>HHHHHHHHMKSESKVSSKLELRELVLLAMVI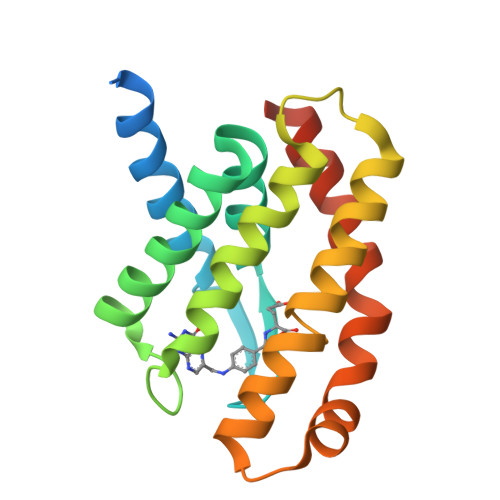AIKVVLGQFKVGDATLQVGLGFIGSVMLGYLFGPWWGFAGGALSDLVSSAIFGNLGGFFIGFTLTAALESMIYGFFLYKKPIQIWRVIASVICVTVICYIGLNTLWVSMLGGTNFMVALSSRILKEMITPWIHMVVVWFILEGLSRVKLSRKF[2x]> GSYAEGQRKRRNTIHEFKKSAKTTLIKIDPALKIKTKKVNTADQCANRCTRNKGLPFTCKAFVFDKARKQCLWFPFNSMSSGVKKEFGHEFDLYENK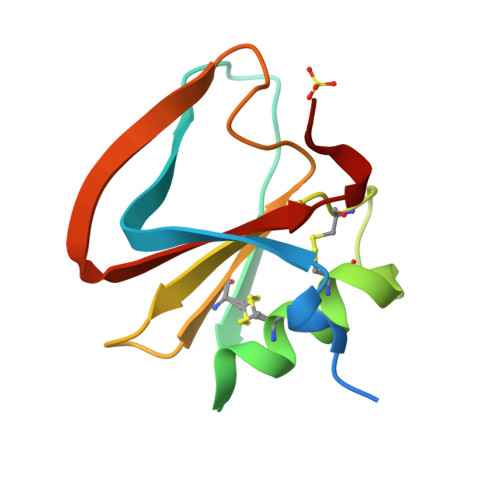DYIR> MIFVLDVGNTNAVLGVFEEGELRQHWRMETDRHKTEDEYGMLVKQLLEHEGLSFEDVKGIIVSSVVPPIMFALERMCEKYFKIKPLVVGPGIKTGLNIKYENPREVGADRIVNAVAGIHLYGSPLIIVDFGT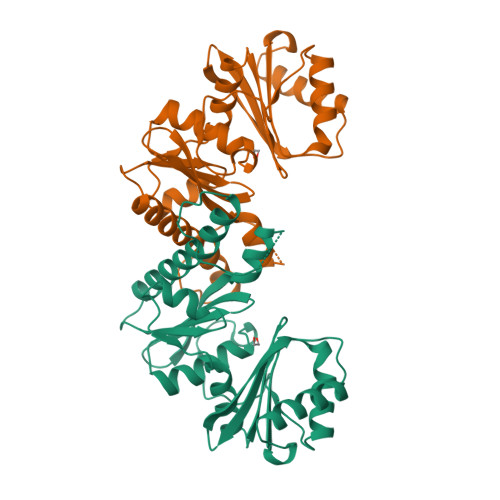ATTYCYINEEKHYMGGVITPGIMISAEALYSRAAKLPRIEITKPSSVVGKNTVSAMQSGILYGYVGQVEGIVKRMKEEAKQEPKVIATGGLAKLISEESNVIDVVDPFLTLKGLYMLYERNANLQHEKGEHHHHHH Protein gradients play a central role in the spatial organization of cells, but the mechanisms of their formation are incompletely understood. This study analyzes the determinants responsible for establishing bipolar gradients of the ATPase MipZ, a key regulator of division site placement in Caulobacter crescentus. MipZ dynamically interacts with the polar ParB-parS complexes, forming a subcellular gradient with concentration maxima at the tips of the cell and a minimum at the cell center. It inhibits polymerization of the tubulin homolog FtsZ into the so-called Z ring, a structure that forms the basis of the bacterial divison apparatus (Erickson et al., 2010). MipZ belongs to the Mrp/MinD family of P loop ATPases, a heterogeneous group of proteins that act as nucleotide-dependent molecular switches (Leipe et al., 2002).

Similar to other Mrp/MinD-type ATPases (Leonard et al., 2005; Schindelin et al., 1997; Wu et al., 2011), MipZ forms a nucleotide “sandwich,” with the ATP-binding sites constituting the core of the dimer interface. In addition, several residues from one subunit form key hydrogen bonds with the nucleotide associated with the other subunit, suggesting that ATP(γS) binding is critical for dimer formation. Consistent with a direct, adaptor-like role of the nucleotide in dimerization, MipZ undergoes only minor conformational changes upon transition from the apo to the ATP-bound state (rmsd of 0.76 Ǻ). Most structural alterations occur in protein regions that contribute to the dimer interface, especially the P loop, the segment ranging from β sheet 5 to helix 6, and the first residues of helix 8, thereby repositioning the side chains critical for intrasubunit interaction. The MipZ dimer displays a central cleft that extends along the subunit interface down to the nucleotide-binding sites, with its bottom being lined by the phosphates of the two nucleotide moieties. The mouth of this cleft is highly negatively charged (bottom, central right). The remaining surface areas of the MipZ dimer, in particular the side across the opening of the cleft (bottom, right), display a high density of positive charges, thus potentially constituting a DNA-binding surface. The first exchange (K13A) targeted Lys13, which contacts the α- and γ-phosphates of the nucleotide bound to the adjacent subunit and might play a key role in both ATP hydrolysis and ATP-dependent dimerization. An additional substitution (G14V) replaced the highly conserved Gly14 in the P loop with a bulky valine residue, causing a steric clash with the γ-phosphate and the Val14 residue of the adjacent subunit that probably also interferes with dimer formation. The third mutation (K18Q) exchanged Lys18, which constitutes an integral part of the nucleotide-binding site, interacting with the β- and γ-phosphates of the nucleotide associated with the cis subunit.

>[2x]MAETRVIVVGNEKGGAGKSTIAVHLVTALLYGGAKVAVIDLALRQRTSARFFENRRAWLDNKKIELPEPLALNLSDNDVALAERPEEEQVAGFEAAFARAMAECDFILIDTPGGDSAITRMAHGRADLVVTPMNDSFVDFDMLGTVDPVTLELTKPSLYSLTVWEGRKQRALSGQRQAMDWVVLRNRLATTEARNRKRLEDRLNALAKRVGFRIGPGLRDRVIYRELFPFGLTIADLSPQVRPVPVSLQHLAARQELRALMHSLGLSAYSGETMLAAQGSHHHHHH Murine Polyomavirus (MuPyV) is a double-stranded DNA virus that can induce tumors in newborn animals. Viral attachment is mediated by the major capsid protein, VP1, which forms pentameric capsomers that assemble into the T = 7d icosahedral capsid of the virus. Sialylated oligosaccharide receptors are engaged in a shallow groove on top of VP1 formed by loop structures on the protein surface, similar to other polyomaviruses. The differences among the three strains have been mapped to amino acid variations at two positions, 91 and 296, within the receptor-binding region of VP1.

The laboratory-derived RA strain shows limited spread and induces few tumors of strictly mesenchymal origin after a long latency period, while the naturally occurring PTA strain has disseminated infection and causes multiple tumors of epithelial and mesenchymal origin within a short time. While RA bears a glycine residue at position 91, this residue is replaced with a glutamate in both PTA and LID. By solving the crystal structures of RA and LID VP1 complexed with GT1a using the identical strategy used for the PTA-GT1a complex, we found that the overall binding mode of GT1a is very similar across the three strains, with a conserved binding mode of the [α-2,8]-linked Neu5Acb. Although the replacement of glutamate with glycine at position 91 leads to a contact area decrease of 33 Å2 in RA, the orientation of GT1a in this strain is not altered (compare Fig 5B and 5C). Due to these steric constraints, the GT1a complexes feature well-defined electron density not only for the binding epitope, but also for the non-binding, branching NeuNAcd in its preferred solution conformation, which brings this moiety to about 5 Å near the end of the long arm and gives the glycan the characteristic, horseshoe-like topology that is observable in all complex structures. The GT1a glycan exhibits the strongest binding in all three VP1 variants compared with DSLNT or GD1a, with no detectable difference between the strains. The stronger overall binding of GT1a can be attributed to the additional [α-2,8]-linked sialic acid present in GT1a (Neu5Acb), which contributes several interactions and an increased buried surface area. These contacts seem to outweigh the differences in van der Waals contacts with the side chains of E91 or V296, at least to the extent discernable in our assay.

>GMEVLDLVTGPDSVTEIEAFLNPRMGQPPTPESLTEGGQYYGWSRGINLATSDTEDSPGNNTLPTWSMAKLQLPMLNEDLTCDTLQMWEAVSVKTEVVGSGSLLDVHGFNKPTDTVNTKGISTPVEGSQYHVFAVGGEPLDLQGLVTDARTKYKEEGVVTIKTITKKDMVNKDQVLNPISKAKLDKDGMYPVEIWHPDPAKNENTRYFGNYTGGTTTPPVLQFTNTLTTVLLDENGVGPLCKGEGLYLSCVDIMGWRVTRNYDVHHWRGLPRYFKITLRKRWVK[5x]Isopentenyl 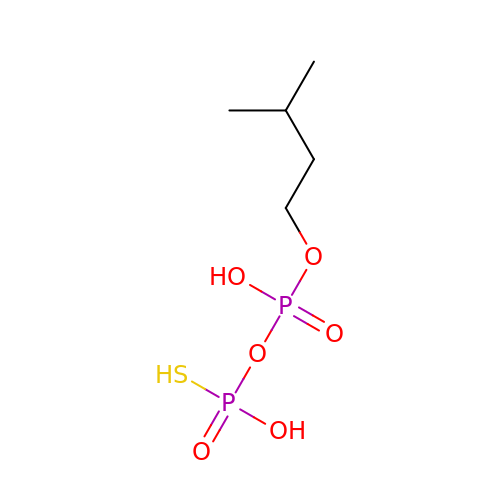Diphosphate Beta-S | C5 H14 O6 P2 S | JPPCYMVZXKAWTF-UHFFFAOYSA-N>[2x]MSEAIVVNNQNDQSRAYAIPLEDIDVSNPELFRDNTMWGYFERLRREDPVHYCKDSLFGPYWSVTKFKDIMQVETHPEI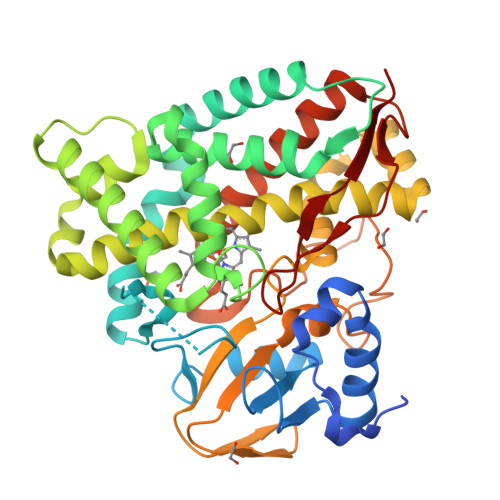FSSEGNITIMESNAAVTLPMFIAMDPPKHDVQRMAVSPIVAPENLAKLEGLIRERTGRALDGLPINETFDWVKLVSINLTTQMLATLFDFPWEDRAKLTRWSDVATALVGTGIIDSEEQRMEELKGCVQYMTRLWNERVNVPPGNDLISMMAHTESMRNMTPEEFLGNLILLIVGGNDTTRNSMTGGVLALNENPDEYRKLCANPALIASMVPEIVRWQTPLAHMRRTALQDTELGGKSIRKGDKVIMWYVSGNRDPEAIENPDAFIIDRAKPRHHLSFGFGIHRCVGNRLAELQLRIVWEELLKRWPNPGQIEVVGAPERVLSPFVKGYESLPVRINA> MSVLQVLHIPDERLRKVAKPVEEVNAEIQRIVDDMFETMYAEEGIGLAATQVDIHQRIIVIDVSENRDERLVLINPELLEKSGETGIEEGCLSIPEQRALVPRAEKVKIRALDRDGKPFEL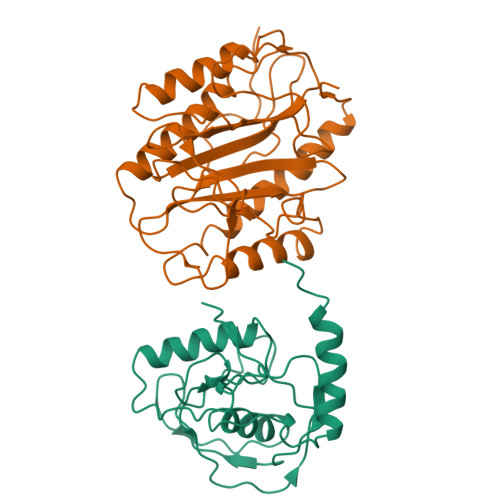EADGLLAICIQHEMDHLVGKLFMDYLSPLKQQRIRQKVEKLDRLKARA;> MAISIKTPEDIEKMRVAGRLAAEVLEMIEPYVKPGVSTGELDRICNDYIVNEQHAVSACLGYHGYPKSVCISINEVVCHGIPDDAKLLKDGDIVNIDVTVIKDGFHGDTSKMFIVGKPTIMGERLCRITQESLYLALRMVKPGINLREIGAAIQKFVEAEGFSVVREYCGHGIGQGFHEEPQVLHYDSRETNVVLKPGMTFTIEPMVNAGKKEIRTMKDGWTVKTKDRSLSAQYEHTIVVTDNGCEILTLRKDDTIPAIISHDE> LESPGFMVHKKLK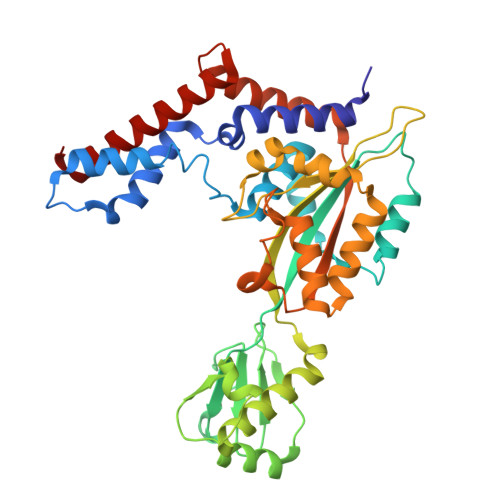SMSQSYGVMMTGVPAEVLGQMQAERSIPSINKTGNLKQQIAKEVSKVCHMMTEPTQSAGQASNDVCELLLGKIEAEKFHFTKYEALSADGDNLKNVLENTAPSSTNLLIRFEIDREDPPIVLVKTKNENFNPETAVKNKIYLLENKLYFIDKMGNLFNLGPGKKKCTQLFNAIGDSAEYSLCDPFVLEEPEKPEDFAISEIVDIFNEQKERFDFWIGSHSFTIYIPQTLGESPRQFYPYQAYFGSHTLQDWFVSDKDEYLSRIGIDKYIEKLAVLGKTTNTKERSDIYAEFFSKRGREAFFCAHLNEKRQPLRVKFKITEINPELALKNLQETQEFIDTHPGENPSDKVENYRNRAKLAMTEHLESLLDI>[2x]GGGSWVCRFYQGKHRGVEVELPHGRCVFGSDPLQSDIVLSDSEIAPVHLVLMVDEEGIRLTDSAEPLLQEGLPVPLGTLLRAGSCLEVGFLLWTFVA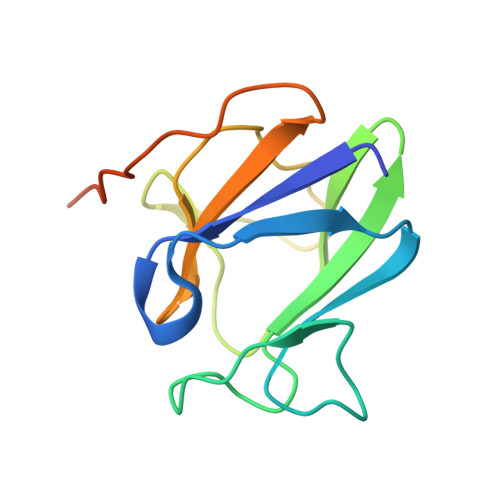VGQPLPETLQVPTQRKEPTDRLPRSR>[3x]MFSKFFIERPIFASVVAIIISIAGIIGLANLPVEQYPSLTPPTVQVS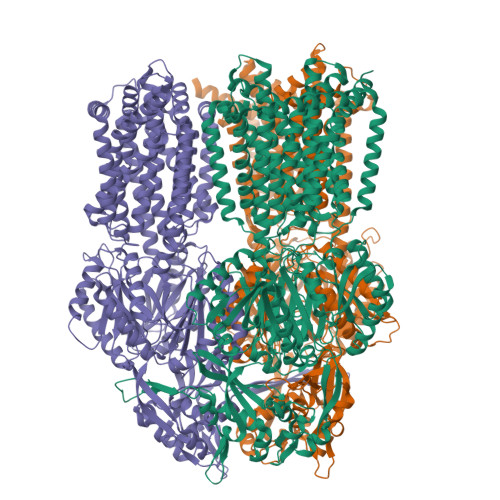ATYTGADAQTIASTVATPIEDAINGVDNMIYMDSTSSPGQMKLTVYFNIGTDPDQAAIDVNNRISAATAKLPEAVKKLGVTVRKSSSTILEVVSVYSEDSSMNDIDIYNYVSLNILDELKRIPGVGDASAIGNKNYSMRIWLEPDLLNKFGVTANDVINAVNDQNAQYATGKIGEEPVVNKSPQVISITMQGRLQTPQEFENIILRVNEDKSFLRIKDVAKVEIGAEQYNSTGRLNTSAAVPIIINLQSGANAVNTAKLINEKMQELSKNFPQGLKYQIPYDTTIFVKASIKEVIKTFVEALALVLVVMYLFLKNFKSTIIPMIAVPVSLLGTFAVLYVLGFSINLLTLFALVLAIGIVVDDAIIVVENIDRILHEDSNISVKDAAIKAMNEVSSPVISIVLVLCAVFIPVSFISGFVGEIQRQFALTLAISVAISGFVALTLTPSLSALFLTRNESKPFYFIQKFNDFFDWSTSVFSSGVAYILKRTIRFVLVFCIMIGFIAYLFKIVPSSLVPSEDQGVIMSIINLPSGSSIHRTIEEVDTINKNATQMKEISSSVSLIGFDLFTSSLKENAAAVFFILKDWSQREASSDQIIAQLFGQYAADRNALSYFLNLPPIPGLSLTGGFEMYAQNKSGKDYDAIQQDVNKMLELARTRKELANVRTTLDTSFPQYKLIIDRDKMKYYNLNMQDVFNTISATIGTYYVNDFPMLGKNFQVNIRALGDFRNTQDALKNIYIRSSDNKMIPLNSFLTLVRSAGPDDVKRFNLFPAALIQGDPAPGYTSGQAIDAIAEVAKQSLGDEYSIAWSGSAYQEVSSKGAGAYAFVLGMIFVFLILAAQYERWLMPLAVITAVPFAVFGSILLVALRGFDNDIYFQTGLLLLIGLSAKNAILIIEFAMEERLKKGKSIFEAAINAAKLRFRPIIMTSLAFTFGVLPMIFATGAGSASRHSLGTGLIGGMIAASTLAIFFVPLFFYLLENFNEWLDKKRGKVHE>[2x]SNATAQQWNKDVVGWNLGNEFECSAPGQDGESMQIGNPDGSIHAETAWGNPVVTKKMIQAVKKAGFNAIRIPIRWQCHITNAQAMSIDKAWIARIKEVVGWCLDNGLKVII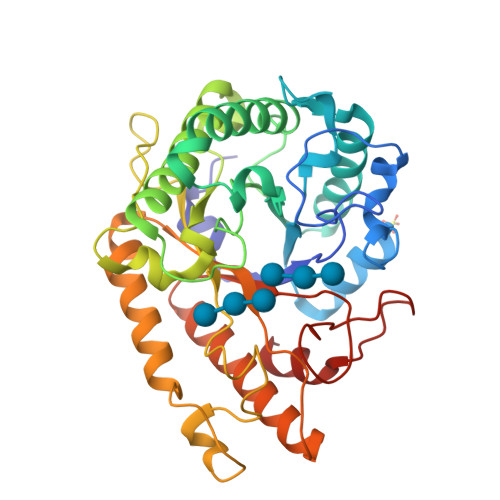NVHHEKWLESRPTYQYKEENCQKLALLWMNIASEFANYDSRLAFAGTNEVHIRDNWGKPTAENLEVQNAYNQIFVDVVRATGGNNAKRHLILQTYVCNPWFGIENGDFIIPKDAEGNGNNYMSVEFHYYQPWSYAGDCTYDYWGDAYKDAGKIPADNEKTMTDFFDKAVNTWSNKGLGIVIGAWGVTDHYKSNSEKVHENMTYYCKFLTTEARKRGFSTFVWDNNHFGNGSEKYGIFDRFKSMKVNAPWILEGIF> MSEQQVQELEKKWYALQVEPGKENEAKENLLKVLELEGLKDLVDEVIVPAEEKVVIRAQGKEKYRLSLKG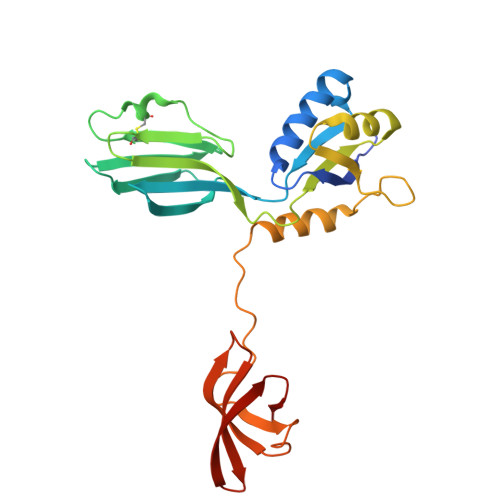NARDISVLGKKGVTTFRIENGEVKVVESVEGDTCVNAPPISKPGQKITCKENKTEAKIVLDNKIFPGYILIKAHMNDKLLMAIEKTPHVFRPVMVGGKPVPLKEEEVQNILNQIKRGVKPSKVEFEKGDQVRVIEGPFMNFTGTVEEVHPEKRKLTVMISIFGRMTPVELDFDQVEKI> MAYENLFLRPACPGNISDTSTYNIDGACVAQGDIGFGSAVQVVGIVDGVKVVAALPDGGTPYGIAFRSQYEHLSGKILDGEVCNVVSHGRVWTLTSLGEAPSLFSKLQFGSGGVVTGGSGSAGWTFAGGFVKHEDGYIIEVQVKQNAFIAPPPPPPVVLVESATIATDKESPQPNNVTIQCVANALPDN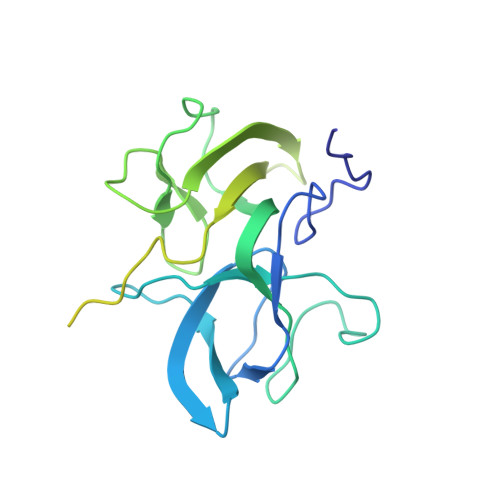ATDKTGKWSIDATNIATVDPDSGLVTPVGGEVVGDFNITWTANDASKTTATIAYRVEAVPTPEVDA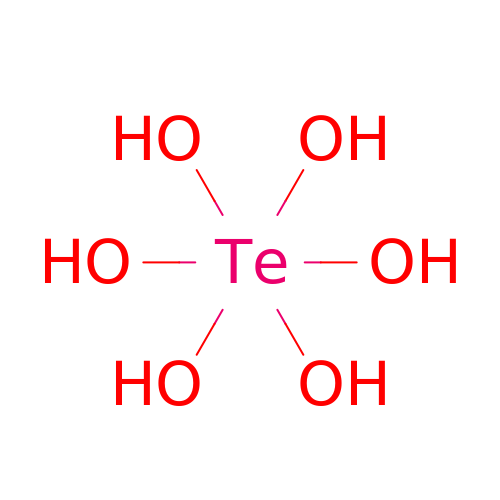Orthotelluric acid | H6 O6 Te | FXADMRZICBQPQY-UHFFFAOYSA-N(3Z)-1-[(6-fluoro-4H-1,3-benzodioxin-8-yl)methyl]-4-[(E)-2-phenylethenyl]-1H-indole-2,3-dione 3-oxime | C25 H19 F N2 O4 | 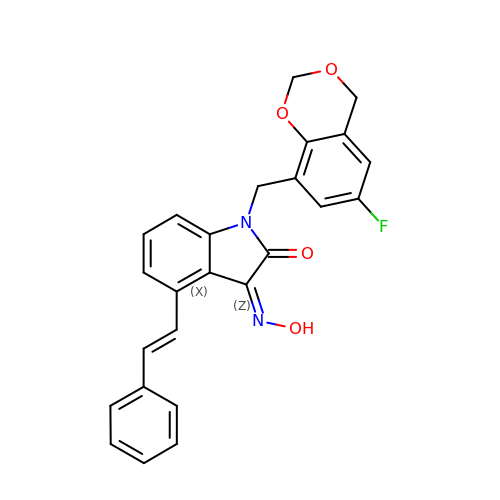DDHASJXGNUWZTM-ZLEWNXFRSA-N> GPLGSMTTTLANRPDGEGSVQVKLDPKVNIEEGALVIAVYGKGGIGKSTTSSNLSAAFSKLGKKVLQIGCDPKHDSTFTLTHKMVPTVIDILEEVDFHSEELRPQDFMFEGFNGVQCVESGGPPAGTGCGGYVTGQTVKLLKEHHLLEDTDVVIFDVLGDVVCGGFAAPLQHANYCLIVTANDFDSIFAMNRIVAAINAKAKNYKVRLGGVIANRSAELDQIEKFNEKTGLKTMAHFRNVDAIRRSRLKKCT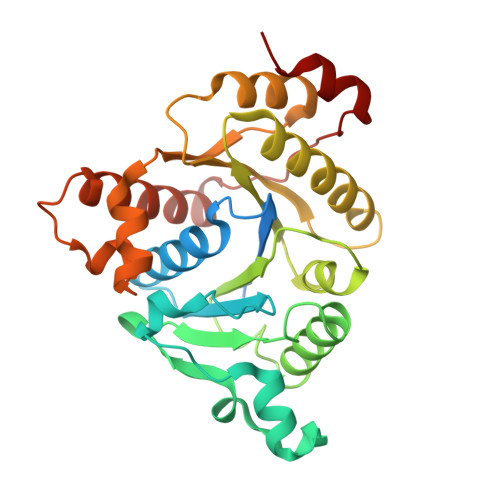IFEMDPEEEGVLEVQNEYLSLAKKMIDNVEPLEAEPLKDREIFDLLGFD>GHMRHIISLLMENEAGALSRVAGLFSARGYNIESLSVAPTEDPTLSRMTLVTNGPDEIVEQITKQLNKLIEVVKLIDLSSEGYVERELMLVKVRAVGKDREEMKRLADIFRGNIIDVTNELYTIELTGTRSKLDGFLQAVDCN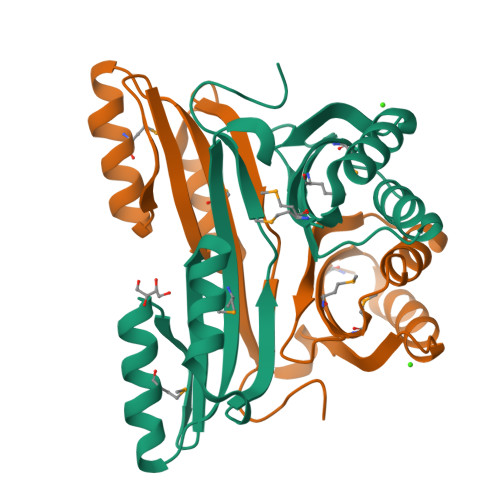LILEIARTGVSGLSRGERVLKL[4x]>[7x]MAIITPALISALKTSFQKH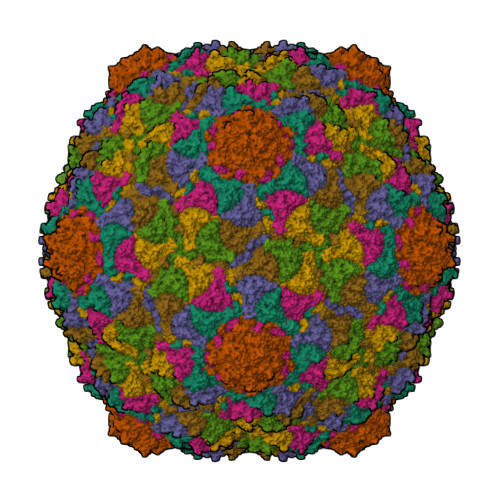FQDALATAPSTYLQVATVIPSTTASNTYGWLGQFPKLREWIGQRVIKDMAAQGYQITNKLFESTVGVKRTDIEDDNLGVYGPLMQEMGRAAGAHPDELVFALLKAGNANLCYDGQNFFDTDHPVYPNVDGTGTATTVSNLFAPAADPGAAWYLLDTSRSLKPLIYQERMKPSFTSMTKEDDEQVFMADEYRYGVRSRCNVGFGFWQLAAMSTEELNQVNFEKVYDAMRNQKADGGRPLDIRPNLLVVPTTLRSKAKEVVGVQRLANGADNPNFELVQVLDTAWLN> GMAEGGAADLDTQRSDIATLLKTSLRK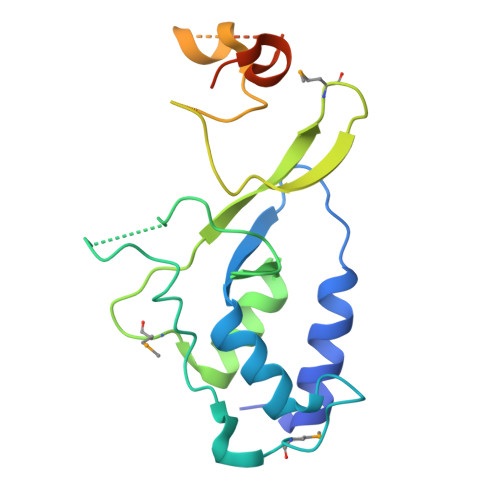GDTWYLVDSRWFKQWKKYVGFDSWDKYQMGDQNVYPGPIDNSGLLKDGDAQSLKEHLIDELDYILLPTEGWNKLVSWYTLMEGQEPIARKVVEQGMFVKHCKVEVYLTELKLCENGNMNNVVTRRFSKADTIDTIEKEIRKIFSIPDEKETRLWNKYMSNTFEPLNKPDSTIQDAGLYQGQVLVIEQKNEDGTWPRG> 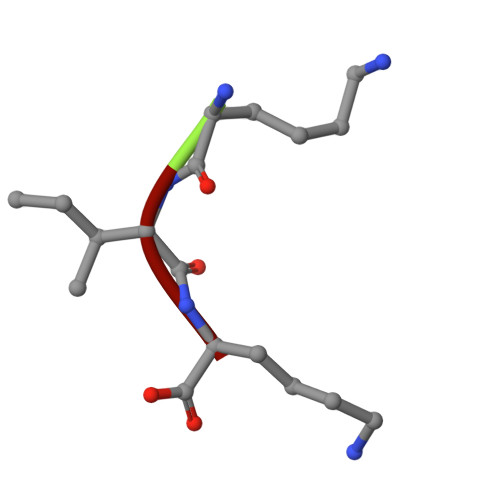KIK2-amino-5-oxo-7-(propan-2-yl)-N-(1H-tetrazol-5-yl)-5H-[1]benzopyrano[2,3-b]pyridine-3-carboxamide | C17 H15 N7 O3 | 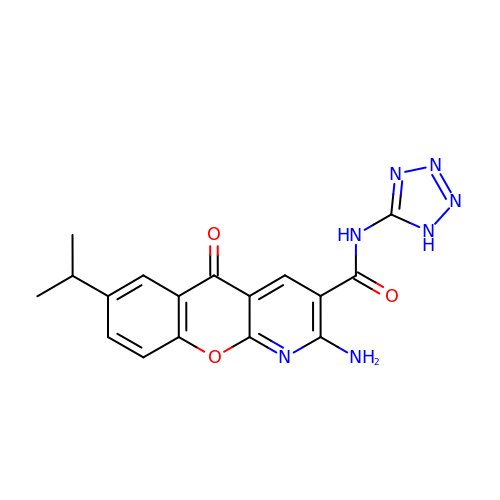JDIHMNISRGRMDY-UHFFFAOYSA-N5-[2-amino-5-(quinolin-3-yl)pyridin-3-yl]-1,3,4-oxadiazole-2(3H)-thione 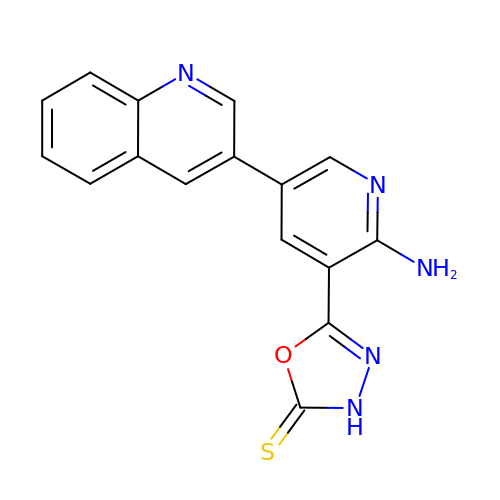| C16 H11 N5 O S | BIPBSLWNCVJIOQ-UHFFFAOYSA-N> MGAPATVTEQGEDITSKKDRGVLKIVKRVGNGEETPMIGDKVYVHYKGKLSNGKKFDSSHDRNEPFVFSLGKGQVIKAWDI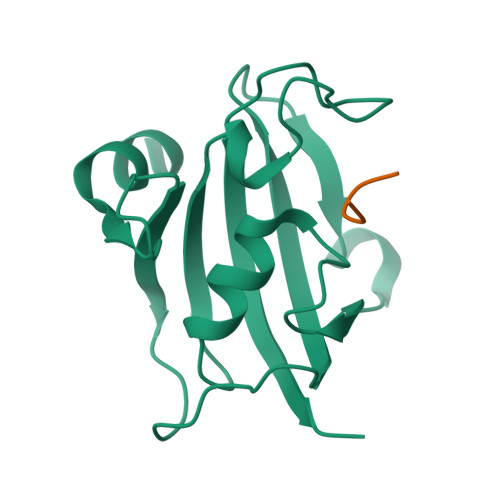GVATMKKGEICHLLCKPEYAYGSAGSLPKIPSNATLFFEIELLDFKGE;> DFPFV>[3x]MMPIKSIVTLDQLEDSEYLFRIVSTVLPHLCLDYKVCDQLKTTFVHPFDILLNNSLGSVTKQDELQAAISKLGINYLIDTTSRELKLFNVTLNAGNIDIINTPINISSETNPIINTHSFYDLPPFTQHLLNIRLTDTEYRARFIGGYIKPDGSDSMDVLAEKKYPDLNFDNTYLFNILYKDVINAPIKEFKAKIVNGVLSRQDF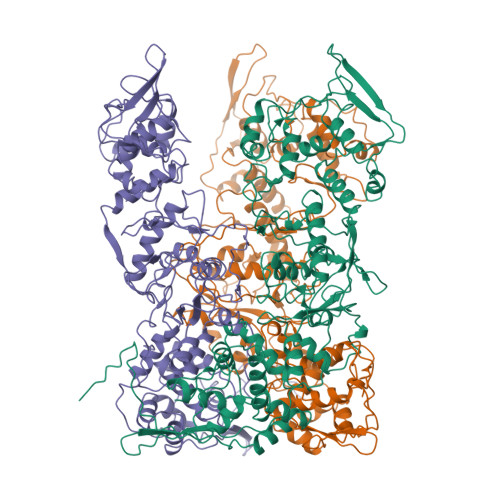DNLIGVRQYITIQDRPRFDDAYNIADAARHYGVNLNTLPLPNVDLTTMPTYKHLIMFEQYFIYTYDRVDIYYNGNKMLFDDEIINFTISMRYQSLIPRLVDFFPDIPVNNNIVLHTRDPQNAAVNVTVALPNVQFVDINRNNKFFINFFNLLAKEQRSTAIKVTKSMFWDGMDYEEYKSKNLQDMMFINSTCYVFGLYNHNNTTYCSILSDIISAEKTPIRVCLLPRVVGGKTVTNLISETLKSISSMTIREFPRKDKSIMHIGLSETGFMRFFQLLRLMADKPHETAIKEVVMAYVGIKLGDKGSPYYIRKESYQDFIYLLFASMGFKVTTRRSIMGSNNISIISIRPRVTKQYIVATLMKTSCSKNEAEKLITSAFDLLNFMVSVSDFRDYQSYRQYRNYCPRYFYAG> ISVCDLPADRGQCTAYIPQWFFAKTTEDCEKFVYGGCQGNANRFETKDDCIANCGCNLPSKVGPCRVSARMWFHNPETEKCEVFIYGGCHGNANRFATETECQEVCDRYQKPGFCYQPSETGPCKGSFPRYYYDYE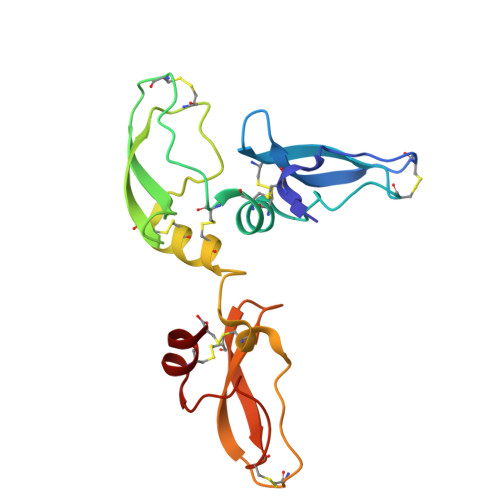DGECKEFIYGGCEGNANNFETKESCENAC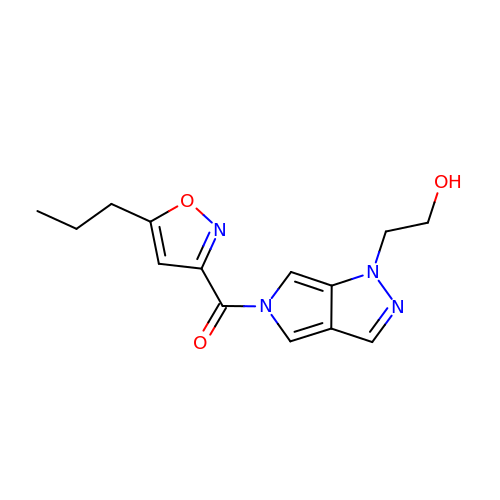[1-(2-hydroxyethyl)pyrrolo[3,4-c]pyrazol-5-yl]-(5-propyl-1,2-oxazol-3-yl)methanone | C14 H16 N4 O3 | NYKTWGKCNASWSV-UHFFFAOYSA-N>AHGGRELIPDEDYWQAVWPNTPIPNTLKELLKPGAQDSEINDVPMKVDDTQYPKTFFFEHELFPGKKMNMKFSKIPFAQPYGVYTWGKVIKDLE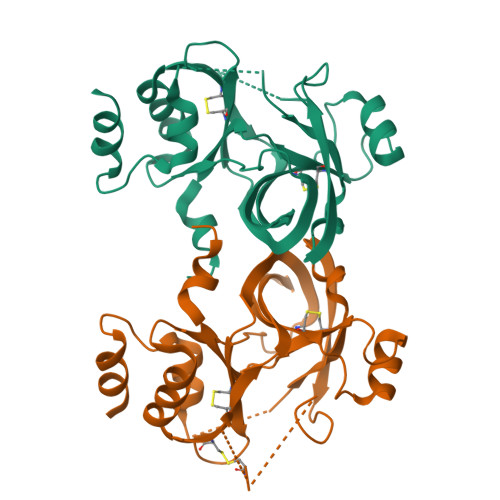KESFTFEDACVREAGKGEDKYCAKSLSTLIGFAVSKLGKNIQPFSSSFLDKQTDYTIEGVHNLGDKAVMCHRLNFQSTVFYCHEIHGTTAYMVPMVAADGRRTQALAVCHHDTSGMNAEVLYEMLKIKPGTETACHFLGNKAVMWVPNMAVNSVYNNANMAS[2x]>MKIFLDTANIDEIRTGVNWGIVDGVTTNPALISKEAVNGKKYGDIIREILKIVDGPVSVEVVSTKYEGMVEEARKIHGLGDNAVVKIPMTEDGLRAIKTLSSEHINTNCTLVFNPIQALLAAKAGVTYVSPFVGRLDDIGEDGMQIIDMIRTIFNNYIIKTQILVASIRNPIHVLRSAVIGADVVTVPFNVLKSLMKHPKTDEGLAK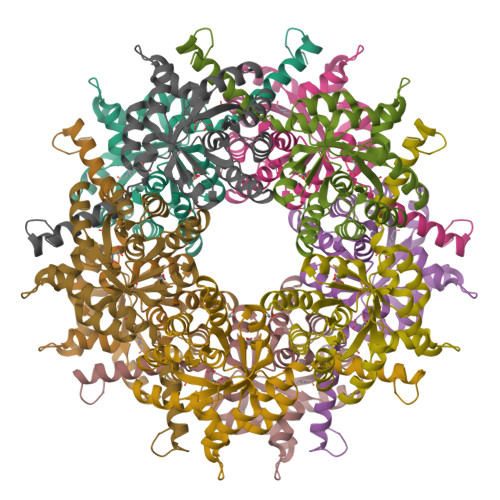FLEDWKKVSPDGKLIL[5x]>[2x]MTADELVFFVNGKKVVEKNADPETTLLAYLRRKLGLRGTKLGCGEGGCGACTVMLSKYDRLQDKIIHFSANACLAPICTLHHVAVTTVEGIGSTKTRLHPVQERIAKSHGSQCGFCTPGIVMSMYTLLRNQPEPTVEEIEDAFQGNLCRCTGYRPILQGFRTFAKNGGCCGGNGNNPNCCMNQKKDHTVTLSPSLFNPEEFMPLDPTQEPIFPPELLRLKDVPPKQLRFEGERVTWIQASTLKELLDLKAQHPEAKLVVGNTEIGIEMKFKNQLFPMIICPAWIPELNAVEHGPEGISFGAACALSSVEKTLLEAVAKLPTQKTEVFRGVLEQLRWFAGKQVKSVASLGGNIITASPISDLNPVFMASGTKLTIVSRGTRRTVPMDHTFFPSYRKTLLGPEEILLSIEIPYSREDEFFSAFKQASRREDDIAKVTCGMRVLFQPGSMQVKELALCYGGMADRTISALKTTQKQLSKFWNEKLLQDVCAGLAEELSLSPDAPGGMIEFRRTLTLSFFFKFYLTVLKKLGKDSKDKCGKLDPTYTSATLLFQKDPPANIQLFQEV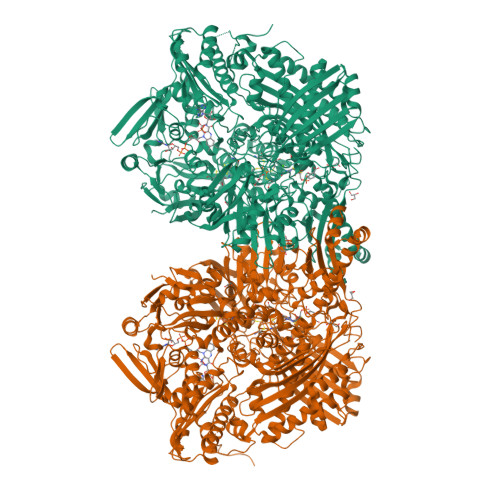PNGQSKEDTVGRPLPHLAAAMQASGEAVYCDDIPRYENELFLRLVTSTRAHAKIKSIDVSEAQKVPGFVCFLSADDIPGSNETGLFNDETVFAKDTVTCVGHIIGAVVADTPEHAERAAHVVKVTYEDLPAIITIEDAIKNNSFYGSELKIEKGDLKKGFSEADNVVSGELYIGGQDHFYLETHCTIAIPKGEEGEMELFVSTQNAMKTQSFVAKMLGVPVNRILVRVKRMGGGFGGKETRSTLVSVAVALAAYKTGHPVRCMLDRNEDMLITGGRHPFLARYKVGFMKTGTIVALEVDHYSNAGNSRDLSHSIMERALFHMDNCYKIPNIRGTGRLCKTNLSSNTAFRGFGGPQALFIAENWMSEVAVTCGLPAEEVRWKNMYKEGDLTHFNQRLEGFSVPRCWDECLKSSQYYARKSEVDKFNKENCWKKRGLCIIPTKFGISFTVPFLNQAGALIHVYTDGSVLVSHGGTEMGQGLHTKMVQVASKALKIPISKIYISETSTNTVPNSSPTAASVSTDIYGQAVYEACQTILKRLEPFKKKNPDGSWEDWVMAAYQDRVSLSTTGFYRTPNLGYSFETNSGNAFHYFTYGVACSEVEIDCLTGDHKNLRTDIVMDVGSSLNPAIDIGQVEGAFVQGLGLFTLEELHYSPEGSLHTRGPSTYKIPAFGSIPTEFRVSLLRDCPNKKAIYASKAVGEPPLFLGASVFFAIKDAIRAARAQHTNNNTKELFRLDSPATPEKIRNACVDKFTTLCVTGAPGNCKPWSLRV>[4x]GHMWQENKSWNAHFTEHKSQGVVVLWNENKQQGFTNNLKRANQAFLPASTFKIPNSLIALDLGVVKDEHQVFK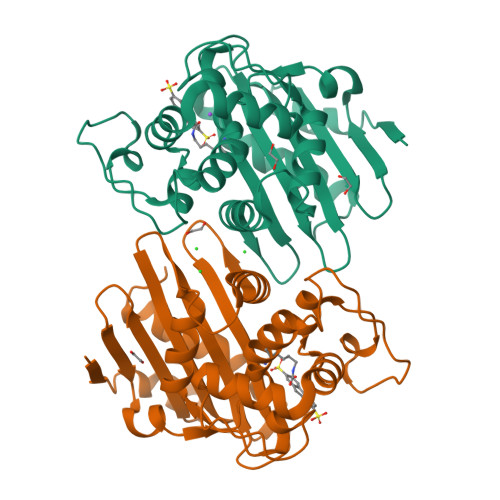WDGQTRDIATWNRDHNLITAMKYSVVPVYQEFARQIGEARMSKMLHAFDYGNEDISGNVDSFWLDGGIRISATEQISFLRKLYHNKLHVSERSQRIVKQAMLTEANGDYIIRAKTGYSTRIEPKIGWWVGWVELDDNVWFFAMNMDMPTSDGLGLRQAITKEVLKQEKIIP Eukaryotes possess eight highly conserved Lsm (like Sm) proteins that assemble into circular, heteroheptameric complexes, bind RNA, and direct a diverse range of biological processes. Among the many essential functions of Lsm proteins, the cytoplasmic Lsm1–7 complex initiates mRNA decay, while the nuclear Lsm2–8 complex acts as a chaperone for U6 spliceosomal RNA. The Sm family includes the Sm, Lsm (“Like Sm”), and bacterial Hfq proteins. These proteins share a conserved “Sm fold” consisting of an amino-terminal alpha helix followed by five antiparallel beta strands that form small beta barrels that assemble into ring-shaped hexamers or heptamers. Here, we elucidate the molecular basis for Lsm-RNA recognition and present four high-resolution structures of Lsm complexes bound to RNAs.

Since deletion of the carboxyl terminus of Lsm1 generally enhances binding affinity, we therefore crystallized the Lsm1Δ56C–7 variant of the Lsm1–7 complex bound to the U-tract RNAs UUUUUA and AUUUUG and determined their structures to resolutions of 1.8 and 2.1 Å, respectively. In the structure of UUUUUA bound to Lsm1Δ56C–7, the first uridine is disordered and not visible in the electron density. The next four uridines occupy pockets in Lsm4, Lsm1, Lsm2, and Lsm3, respectively. The terminal adenosine reaches across Lsm6 to form a hydrogen bond to Asn66 of Lsm5. This is the first observation of Lsm5 interacting with RNA; Lsm5 is not utilized in the Lsm2–8 structures. Furthermore, Lsm5 is the only Lsm protein out of the eight studied here that has a noncanonical nucleobase binding pocket because it is missing the arginine that typically forms a cation-pi stack with uracil (Zhou et al. 2014a,b; Montemayor et al. 2018). In place of arginine, Lsm5 has an asparagine (Asn66) that forms a hydrogen bond to the terminal adenine. We further tested the effect of 3′-end nucleotide identity on binding and found that tetrauridylate followed by a single adenosine binds more tightly than an RNA with a pentauridylate tract. The trajectory of the RNA in Lsm1Δ56C–7 suggests that the RNA can thread completely through the ring, provided the Lsm1 carboxy-terminal helix is removed or displaced.

> GSMNQATQIIPFTTSGSLVDYVDRKVIVVLRDGKKLIGILRSFDQFANLMLQYTIERIYVDDMYGDIDRGVYIVRGENVVLLGELD;> MLFYSFFKTLIDTEVTVELKNDMSIRGILKSVDQFLNVKLENISVVDASKYPHMAAVKDLFIRGSVVRYVHMSSAYVDTILLADACRRDLANNKRQ;> GSMESAQAVAEPLDLVRLSLDEIVYVKLRGDRELNGRLHAYDEHLNMVLGDAEEIVTIFDDEETDKDKALKTIRKHYEMLFVRGDSVILIAPPRN;> MLPLTLLNATQGRPILVELKNGETFNGHLENCDNYMNLTLREVIRTMPDGDKFFRLPECYIRGNNIKYLRIQDEVLSQVAKQQAQQRENRGSRFRGRGQRGRGNYGHTAPNRRGRGRGGHMWSHPQFEK;> MSMTILPLELIDKCIGSNLWVIMKSEREFAGTLVGFDDYVNIVLKDVTEYDTVTGVTEKHSEMLLNGNGMCMLIPGGKPE;> GSMDSSPNEFLNKVIGKKVLIRLSSGVDYKGILSCLDGYMNLALERTEEYVNGKKTNVYGDAFIRGNNVLYVSALDD;> MSSLQKRPGPGNSSQPTERPRKESILDLSRYQDQRIQATFTGGRQITGILKGFDQLMNLVLDDVEEQLRNPEDGKLTGAIRKLGLVVVRGTTLVLIAPMDGSEEIPNPFVQAEHHHHHH> FMVSLPRMVYPQPKVLTPCRKDVLVVTPWLAPIVWEGTFNIDILNEQFRLQNTTIGLTVFAIKKYVAFLKLFLETAEKHFMVGHRVHYYVFTDQPAAVPRVTLGTGRQLSVLEVGAYKRWQDVSMRKMEMISDFCER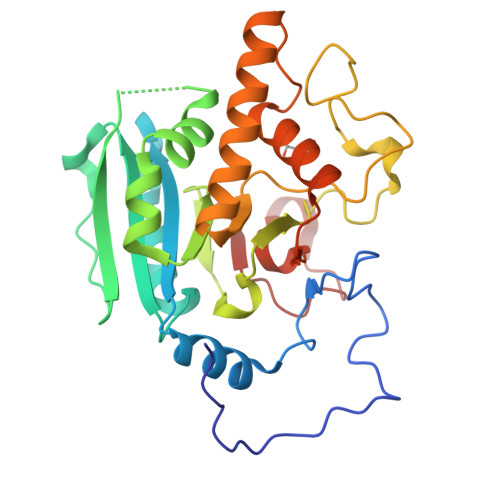RFLSEVDYLVCVDVDMEFRDHVGVEILTPLFGTLHPSFYGSSREAFTYERRPQSQAYIPKDEGDFYYMGAFFGGSVQEVQRLTRACHQAMMVDQANGIEAVWHDESHLNKYLLRHKPTKVLSPEYLWDQQLLGWPAVLRKLRFTAVP>SMPKPIYSYSILIFMALKNSKTGSLPVSEIYNFMTEHFPYFKTAPDGWKNSVRHNLSLNKCFEKVENKSG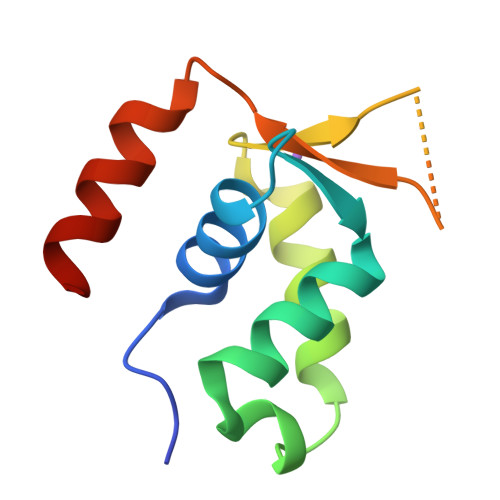SSSRKGCLWALNPAKIDKMQEELQKWKRK[8x]> GPLGSEQLKCCSGILKEMFAKKHAAYAWP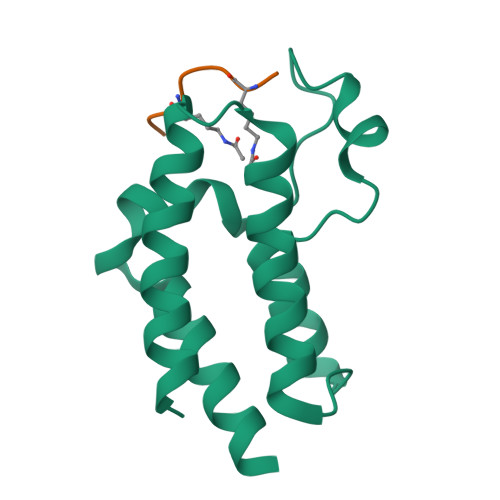FYKPVDVEALGLHDYCDIIKHPMDMSTIKSKLEAREYRDAQEFGADVRLMFSNCYKYNPPDHEVVAMARKLQDVFEMRFAKM;> GKAGKDS>MGADRRGERMNLEQHAGARAPNTSSSRPKTLLVKHADVLVTMDDTRRELRDAGLYIEDNRIVAVGPSAELPETADEVLDLRGHLVIPGLVNTHHHMYQSLTRAVPAAQNAELFGWLTNLYKIWAHLTPEMIEVSTLTAMAELLQSGCTTSSDHLYIYPNGSRLDDSIGAAQRIGMRFHASRGAMSVGQRDGGLPPDSVVEREPDILRDTQRLIETYHDEGRYAMLRVVVAPCSPFSVSRDLMRDAAVLAREYGVSLHTHLAENVNDIAYSREKFGMTPAEYAEDLGWVGHDVWHAHCVQLDDAGIGLFARTGTGVAHCPCSNMRLASGIAPVKKMRLAGVPVGLGVDGSASNDGAQMVAEVRQALLLQRVGFGPDAMTAREALEIATLGGAKVLNRDDIGALKPGMAADFAAFD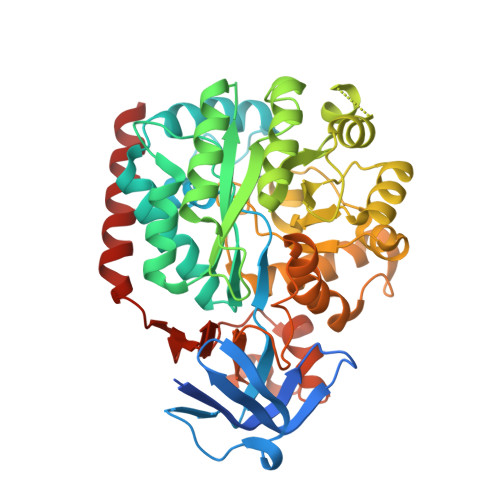LRQPLFAGALHDPVAALVFCAPSQTAYTVVNGKVVVREGRLATLDLPPVIERHNALAHALVEAAR[2x]> MRGSHHHHHHGSEEASSTGRNFNVEKINGEWHTIILASDKREKIEDNGNFRLFLEQIHVLEKSLVLKFHGRVRLLNNWDCSELSMV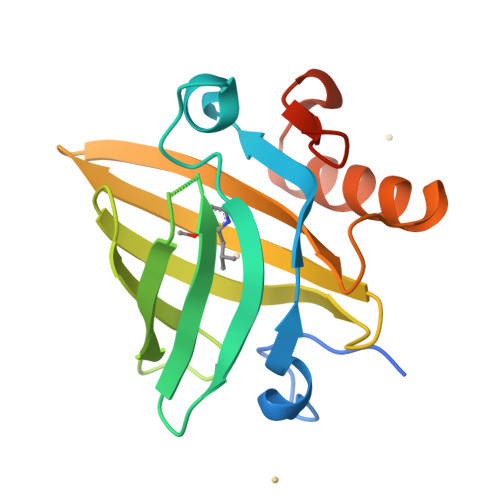ADKTEKAGEYSVTYDGFNTFTIPKTDYDNFLMAHLINEKDGETFQLMGLYGREPDLSSDIKERFAQLCEEHGILRENIIDLSNANRCLQARE>MSLKHYSIQPANLEFNAEGTPVSRDFDDVYFSNDNGLEETRYVFLG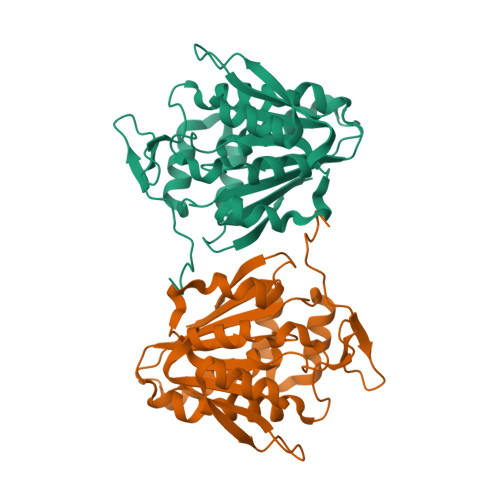GNQLEARFPEHPHPLFVVAESGFGTGLNFLTLWQAFDQFREAHPQAQLQRLHFISFEKFPLTRADLALAHQHWPELAPWAEQLQAQWPMPLPGCHRLLLDEGRVTLDLWFGDINELISQLDDSLNQKVDAWFLDGFAPAKNPDMWTQNLFNAMARLARPGGTLATFTSAGFVRRGLQEAGFTMQKRKGFGRKREMLCGVMEQTEGHHHHHH[2x]> GDIFYPGYCPDVKPVNDFDLSAFAGAWHEIAKLPLENENQGKCTIAEYKYDGKKASVYNSFVSNGVKEYMEGDLEIAPDAKYTKQGKYVMTFKFGQRVVNLVPWVLATDYKNYAINY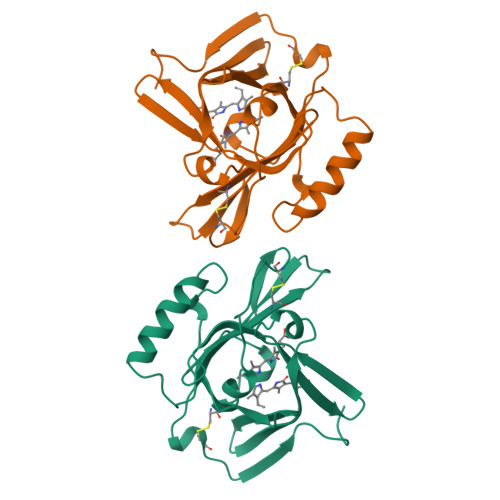NCDYHPDKKAHSIHAWILSKSKVLEGNTKEVVDNVLKTFSHLIDASKFISNDFSEAACQYSTTYSLTGPDRH> MLGTGPAAATTAATTSXXXXXXXXXXXXXXSRNEETXXXXXXXXXXXXXXXXXEMSQEEXTRFYDQLNHHIFELVSSSDANERKGGILAIASLIGVEGGNATRIGRFANYLRNLLPSNDPVVMEMASKAIGRLAMAGDTFTAEYVEFEVKRALEWLGADRNEGRRHAAVLVLRELAISVPTFFFQQVQPFFDNIFVAVWDPKQAIREGAVAALRACLILTTQREPKEMQKPQWYRHTFEEAEKGFDETLAKEKGMNRDDRIHGALLILNELVRISSMEGERLREEMEEITQQQLVHDKYCKDLMGFGTKPRHITPFTSFQAVQPQQSNALVGLLGYSSHQGLMGFGTSPSPAKSTXXXXXXXXXXXXXXXXXXXXXXXKCRNSKNSLIQMTILNLLPRLAAFRPSAFTDTQYLQDTMNHVLSCVKKEKERTAAFQALGLLSVAVRSEFKVYLPRVLDIIRAALPPKDFAHKRQKAMQVDATVFTCISMLARAMGPGIQQDIKELLEPMLAVGLSPALTAVLYDLSRQIPQLKKDIQDGLLKMLSLVLMHKPLRHPGMPKGLAHQLASPGLTTLPEASDVGSITLALRTLGSFEFEGHSLTQFVRHCADHFLNSEHKEIRMEAARTCSRLLTPSIHLISGHAHVVSQTAVQVVADVLSKLLVVGITDPDPDIRYCVLASLDERFDAHLAQAENLQALFVALNDQVFEIRELAICTVGRLSSMNPAFVMPFLRKMLIQILTELEHSGIGRIKEQSARMLGHLVSNAPRLIRPYMEPILKALILKLKDPDPDPNPGVINNVLATIGELAQVSGLEMRKWVDELFIIIMDMLQDSSLLAKRQVALWTLGQLVASTGYVVEPYRKYPTLLEVLLNFLKTEQNQGTRREAIRVLGLLGALDPYKHKVNIGMIDQSRDASAVSLSESKSSQDSSDYSTSEMLVNMGNLPLDEFYPAVSMVALMRIFRDQSLSHHHTMVVQAITFIFKSLGLKCVQFLPQVMPTFLNVIRVCDGAIREFLFQQLGMLVSFVKSHIRPYMDEIVTLMREFWVMNTSIQSTIILLIEQIVVALGGEFKLYLPQLIPHMLRVFMHDNSPGRIVSIKLLAAIQLFGANLDDYLHLLLPPIVKLFDAPEAPLPSRKAALETVDRLTESLDFTDYASRIIHPIVRTLDQSPELRSTAMDTLSSLVFQLGKKYQIFIPMVNKVLVRHRINHQRYDVLICRIVKGYTLADEEEDPLIYQHRMLRSGQGDALASGPVETGPMKKLHVSTINLQKAWGAARRVSKDDWLEWLRRLSLELLKDSSSPSLRSCWALAQAYNPMARDLFNAAFVSCWSELNEDQQDELIRSIELALTSQDIAEVTQTLLNLAEFMEHSDKGPLPLRDDNGIVLLGERAAKCRAYAKALHYKELEFQKGPTPAILESLISINNKLQQPEAAAGVLEYAMKHFGELEIQATWYEKLHEWEDPLVAYDKKMDTNKDDPELMLGRMRCLEALGEWGQLHQQCCEKWTLVNDETQAKMARMAAAAAWGLGQWDSMEEYTCMIPRDTHDGAFYRAVLALHQDLFSLAQQCIDKARDLLDAELTAMAGESYSRAYGAMVSCHMLSELEEVIQYKLVPERREIIRQIWWERLQGCQRIVEDWQKILMVRSLVVSPHEDMRTWLKYASLCGKSGRLALAHKTLVLLLGVDPSRQLDHPLPTVHPQVTYAYMKNMWKSARKIDAFQHMQHFVQTMQQQAQHAIATEDQQHKQELHKLMARCFLKLGEWQLNLQGINESTIPKVLQYYSAATEHDRSWYKAWHAWAVMNFEAVLHYKHQNQARDEKKKLRHASGANITNATTAATTAATATTTASTEGSNSESEAESTENSPTPSPLQKKVTEDLSKTLLMYTVPAVQGFFRSISLSRGNNLQDTLRVLTLWFDYGHWPDVNEALVEGVKAIQIDTWLQVIPQLIARIDTPRPLVGRLIHQLLTDIGRYHPQALIYPLTVASKSTTTARHNAANKILKNMCEHSNTLVQQAMMVSEELIRVAILWHEMWHEGLEEASRLYFGERNVKGMFEVLEPLHAMMERGPQTLKETSFNQAYGRDLMEAQEWCRKYMKSGNVKDLTQAWDLYYHVFRRISKQLPQLTSLELQYVSPKLLMCRDLELAVPGTYDPNQPIIRIQSIAPSLQVITSKQRPRKLTLMGSNGHEFVFLLKGHEDLRQDERVMQLFGLVNTLLANDPTSLRKNLSIQRYAVIPLSTNSGLIGWVPHCDTLHALIRDYREKKKILLNIEHRIMLRMAPDYDHLTLMQKVEVFEHAVNNTAGDDLAKLLWLKSPSSEVWFDRRTNYTRSLAVMSMVGYILGLGDRHPSNLMLDRLSGKILHIDFGDCFEVAMTREKFPEKIPFRLTRMLTNAMEVTGLDGNYRITCHTVMEVLREHKDSVMAVLEAFVYDPLLNWRLMDTNTKGNKRSRTRTDSYSAGQSVEILDGVELGEPAHKKTGTTVPESIHSFIGDGLVKPEALNKKAIQIINRVRDKLTGRDFSHDDTLDVPTQVELLIKQATSHENLCQCYIGWCPFW;> MNTSPGTVGSDPVILATAGYDHTVRFWQAHSGICTRTVQHQDSQVNALEVTPDRSMIAAAGYQHIRMYDLNSNNPNPIISYDGVNKNIASVGFHEDGRWMYTGGEDCTARIWDLRSRNLQCQRIFQVNAPINCVCLHPNQAELIVGDQSGAIHIWDLKTDHNEQLIPEPEVSITSAHIDPDASYMAAVNSTGNCYVWNLTGGIGDEVTQLIPKTKIPAHTRYALQCRFSPDSTLLATCSADQTCKIWRTSNFSLMTELSIKSGNPGESSRGWMWGCAFSGDSQYIVTASSDNLARLWCVETGEIKREYGGHQKAVVCLAFNDSVLG;> MEEGGSTGSAGSDSSTSGSGGAQQRELERMAEVLVTGEQLRLRLHEEKVIKDRRHHLKTYPNCFVAKELIDWLIEHKEASDRETAIKLMQKLADRGIIHHVCDEHKEFKDVKLFYRFRKDDGTFPLDNEVKAFMRGQRLYEKLMSPENTLLQPREEEGVKYERTFMASEFLDWLVQEGEATTRKEAEQLCHRLMEHGIIQHVSSKHPFVDSNLLYQFRMNFRRRRRLMELLNEKSPSSQETHDSPFCLRKQSHDNRKSTSFMSVSPSKEIKIVSAVRRSSMSSCGSSGYFSSSPTLSSSPPVLCNPKSVLKRPVTSEELLTPGAPYARKTFTIVGDAVGWGFVVRGSKPCHIQAVDPSGPAAAAGMKVCQFVVSVNGLNVLHVDYRTVNNLILTGPRTIVMEVMEELEC;> MESEMLQSPLLGLGEEDEADLTDWNLPLAFMKKRHCEKIEGSKSLAQSWRMKDRMKTVSVALVLCLNVGVDPPDVVKTTPCARLECWIDPLSMGPQKALETIGANLQKQYENWQPRARYKQSLDPTVDEVKKLCTSLRRNAKEERVLFHYNGHGVPRPTVNGEVWVFNKNYTQYIPLSIYDLQTWMGSPSIFVYDCSNAGLIVKSFKQFALQREQELEVAAINPNHPLAQMPLPPSMKNCIQLAACEATELLPMIPDLPADLFTSCLTTPIKIALRWFCMQKCVSLVPGVTLDLIEKIPGRLNDRRTPLGELNWIFTAITDTIAWNVLPRDLFQKLFRQDLLVASLFRNFLLAERIMRSYNCTPVSSPRLPPTYMHAMWQAWDLAVDICLSQLPTIIEEGTAFRHSPFFAEQLTAFQVWLTMGVENRNPPEQLPIVLQVLLSQVHRLRALDLLGRFLDLGPWAVSLALSVGIFPYVLKLLQSSARELRPLLVFIWAKILAVDSSCQADLVKDNGHKYFLSVLADPYMPAEHRTMTAFILAVIVNSYHTGQEACLQGNLIAICLEQLNDPHPLLRQWVAICLGRIWQNFDSARWCGVRDSAHEKLYSLLSDPIPEVRCAAVFALGTFVGNSAERTDHSTTIDHNVAMMLAQLVSDGSPMVRKELVVALSHLVVQYESNFCTVALQFIEEEKNYALPSPATTEGGSLTPVRDSPCTPRLRSVSSYGNIRAVATARSLNKSLQNLSLTEESGGAVAFSPGNLSTSSSASSTLGSPENEEHILSFETIDKMRRASSYSSLNSLIGVSFNSVYTQIWRVLLHLAADPYPEVSDVAMKVLNSIAYKATVNARPQRVLDTSSLTQSAPASPTNKGVHIHQAGGSPPASSTSSSSLTNDVAKQPVSRDLPSGRPGTTGPAGAQYTPHSHQFPRTRKMFDKGPEQTADDADDAAGHKSFISATVQTGFCDWSARYFAQPVMKIPEEHDLESQIRKEREWRFLRNSRVRRQAQQVIQKGITRLDDQIFLNRNPGVPSVVKFHPFTPCIAVADKDSICFWDWEKGEKLDYFHNGNPRYTRVTAMEYLNGQDCSLLLTATDDGAIRVWKNFADLEKNPEMVTAWQGLSDMLPTTRGAGMVVDWEQETGLLMSSGDVRIVRIWDTDREMKVQDIPTGADSCVTSLSCDSHRSLIVAGLGDGSIRVYDRRMALSECRVMTYREHTAWVVKASLQKRPDGHIVSVSVNGDVRIFDPRMPESVNVLQIVKGLTALDIHPQADLIACGSVNQFTAIYNSSGELINNIKYYDGFMGQRVGAISCLAFHPHWPHLAVGSNDYYISVYSVEKRVR

The mammalian/mechanistic target of rapamycin complex 1 (mTORC1) is a large (~1 MDa) multiprotein complex consisting of two copies of three subunits: the evolutionary conserved Serine/Threonine protein kinase mTOR (a member of the phosphoinositide-3-kinase-related kinases superfamily of protein kinases, PIKKs), RAPTOR and mLST8. mTORC1 senses and integrates inputs originating from nutrients, growth factor signaling pathways, oxidative stress, and cellular energy levels. Two endogenous negative regulators of mTORC1 activity have been identified to date: DEPTOR (DEP-domain containing mTOR-interacting protein), which also inhibits mTORC2, and PRAS40 (proline-rich Akt substrate of 40 kDa). DEPTOR is a 46 kDa protein that consists of three distinct and highly conserved regions (from N- to C-terminus): two tandem DEP domains (a DEPt), an unstructured linker of ~100 residues (residues 228–323, which we have named long-linker) and a C-terminal PDZ domain. Our structural and functional analysis of reconstituted mTORC1 inhibition by DEPTOR revealed a unique bipartite binding mechanism, involving an interaction of the DEPTOR PDZ with the FAT domain of mTOR and the DEPTOR long-linker interaction with the FRB.

A similar reduction in DEPTOR IC50 was observed for the cancer-associated mTOR mutant A1459P. The cancer-associated mutant A1459P is in the middle of a helix fα12 at the major intra-FAT hinge, and our cryo-EM structure of the A1459P mutant bound to DEPTOR (global resolution 4.7 Å) shows this helix becomes disordered (residues 1457–1470). This disorder likely increases plasticity of the intra-FAT hinge, thereby improving DEPTOR binding. The structure of mutant mTORC1 bound to DEPTOR reveals a widening of the cleft between the mTOR N-heat and the PDZ-bound FAT domain, relative to this cleft in the structure of DEPTOR bound to wild-type mTORC1. This cleft widening might enable easier access for DEPTOR PDZ to bind to the FAT domain. Consistent with this proposal, we observe fast on/off kinetics for PDZ binding to the mTORC1 mutant A1459P with a Kd of 0.6 µM determined by SPR. For the wild-type mTORC1, the Kd is increased ten-fold (Kd = 7 µM), and we observe slow on/off kinetics, which suggests that there is a rate-limiting conformational change within wild-type mTOR to facilitate binding of PDZ. Structurally, the interaction of DEPTOR PDZ with the FAT domain does not seem to be significantly altered between mutant and wild-type mTORC1. Despite tight binding of DEPTOR PDZ to the A1459P mutant, there is no inhibition of the mutant by the isolated PDZ domain (without the long linker), even at saturating concentrations. This underlines the need for a bipartite interaction for effective mTORC1 inhibition by DEPTOR.The heterotrimeric [FeFe] hydrogenase, HydABC, from T. maritima is a soluble cytoplasmic enzyme involved in fermentation. It uses electrons from the one-electron carrier ferredoxin (E°′ ≈ −450 mV Schut and Adams, 2009), which is reduced during pyruvate metabolism, and the two-electron carrier NADH (E°′ ≈ −20 mV; Schut and Adams, 2009), produced during glucose metabolism, to reduce protons to hydrogen (E°′ ≈ −420 mV; Schut and Adams, 2009). The electron-bifurcating [FeFe] hydrogenase from Thermotoga maritima (HydABC) requires both NADH and ferredoxin to reduce protons generating hydrogen. Electron bifurcation is a fundamental energy conservation mechanism in nature in which two electrons from an intermediate-potential electron donor are split so that one is sent along a high-potential pathway to a high-potential acceptor and the other is sent along a low-potential pathway to a low-potential acceptor.

Following grid imaging, data collection, and processing, we obtained a 2.3-Å resolution map when D2 symmetry was enforced. The processed cryo-EM map shows that HydABC forms a dodecameric complex, Hyd(ABC)4, composed of a tetramer of HydABC heterotrimer units (from now on referred to as protomers). Oligomerization of HydABC occurs through interactions between four HydA subunits in the core of the complex. The HydA core is the best resolved part of the map, consistent with the core being rigid and homogenous. Based on the density map, each HydABC protomer appears to contain nine redox cofactors including five [4Fe–4S] clusters (one of which forms the [4Fe–4S] subcluster of the H-cluster), three [2Fe–2S] clusters, and one FMN. Initially, the last 91 and 61 CT residues of HydA and HydB, respectively, could not be built as they were not present in the homology model (because complex I does not contain homologous domains) and had a low resolution in the map, indicating regions of high heterogeneity (explored later). Electron transfer chains, often connecting distant active sites, are composed of redox-active cofactors usually less than 14 Å apart to allow sufficiently fast electron tunneling through the protein dielectric to sustain physiological processes. In each HydABC heterotrimer, the spatially distant H-clusters and FMN centers are connected via a chain of four FeS clusters (A1, A2, A3, and B2, see Figure 1D for cluster nomenclature). The two tightly interacting HydABC protomers within the Hyd(ABC)2 unit are connected (8.8 Å separation) through the His-ligated [4Fe–4S] cluster (A4) in HydA, part of the so-called Y-junction of iron–sulfur clusters. Within the Hyd(ABC)4 complex, there appear to be two redox networks, each composed of two HydABC protomers with an extended electron transfer chain, separated by at least 50 Å and held together by extensive HydA–HydA interactions.

>[4x]MKIYVDGREVIINDNERNLLEALKNVGIEIPNLCYLSEASIYGACRMCLVEINGQITTSCTLKPYEGMKVKTNTPEIYEMRRNILELILATHNRDCTTCDRNGSCKLQKYAEDFGIRKIRFEALKKEHVRDESAPVVRDTSKCILCGDCVRVCEEIQGVGVIEFAKRGFESVVTTAFDTPLIETECVLCGQCVAYCPTGALSIRNDIDKLIEALESDKIVIGMIAPAVRAAIQEEFGIDEDVAMAEKLVSFLKTIGFDKVFDVSFGADLVAYEEAHEFYERLKKGERLPQFTSCCPAWVKHAEHTYPQYLQNLSSVKSPQQALGTVIKKIYARKLGVPEEKIFLVSFMPCTAKKFEAEREEHEGIVDIVLTTRELAQLIKMSRIDINRVEPQPFDRPYGVSSQAGLGFGKAGGVFSCVLSVLNEEIGIEKVDVKSPEDGIRVAEVTLKDGTSFKGAVIYGLGKVKKFLEERKDVEIIEVMACNYGCVGGGGQPYPNDSRIREHRAKVLRDTMGIKSLLTPVENLFLMKLYEEDLKDEHTRHEILHTTYRPRRRYPEKDVEILPVPNGEKRTVKVCLGTSCYTKGSYEILKKLVDYVKENDMEGKIEVLGTFCVENCGASPNVIVDDKIIGGATFEKVLEELSKNG;>[4x]MFKNAKEFVQYANKLKTLREKKLNGVSIYVCVGTGCTAKGALKVYSAFEEELKKRNLLGQVTLEKIDDDKVTLNRTGCCGRCSSGPLVKIMPYRFFYSNVAPEDVPEIVDRTVLKGEPIERLFLTDPLTGEKVPRIEDTTLFKNQDFYIMEAIGESECDSIEDYIARSGYESLVKALTSMTPEEIIETVKASGLRGRGGGGFPTGLKWEFTRKAQGDIKFVVCNGDEGDPGAFMNRTLLERDPHLVLEGMIIAGYAVGAQKGYAYIRAEYPFAVKMFKKAIEDARKLGLLGENILGTGFSFDLEVKEGAGAFVCGEETALLASIEGKRGMPRPKPPFPAQSGLWGKPTLINNVETYANIPRILRDGVENYRKRGTENSPGTKMFSVAGPLKATGIIEVEFGTTLRDIIYNICGGFVEGEEFKAVQIGGPSGACLSEDFIDMPLDYDTLKKADAMVGSGGIVVITKKTCMVEVARFFLDFTKRESCGKCVPCREGTMQAYNILEKFTHGKATYEDLKTLEHLSKTIKTASLCGLGKTAPNPILSTLKLFREEYIAHIEGECPSGMCTAFKKYVINPDICKGCGLCARSCPQNAITGERGKPYTIDQEKCVKCGLCASKCPFKAIELV;>[4x]MASWSHPQFEKSGGGGGENLYFQGAVLALERHFEKVEEILKKYGYKRENLIKILLEIQEIYRYLPEDVINYVSTAMGIPPAKIYGVATFYAQFSLKPKGKYTIMVCDGTACHMAGSPEVLKAIEEETGLTPGNVTEDLMFSLDQVGCLGACALAPVMVINGEVYGNLTADKVKEILRKIKEKERESANV> GPGSIPDYQEQDIFLWRKETGFGFRILGGNEPGEPIYIGHIVPLGAADTDGRLRSGDELICVDGTPVIGKSH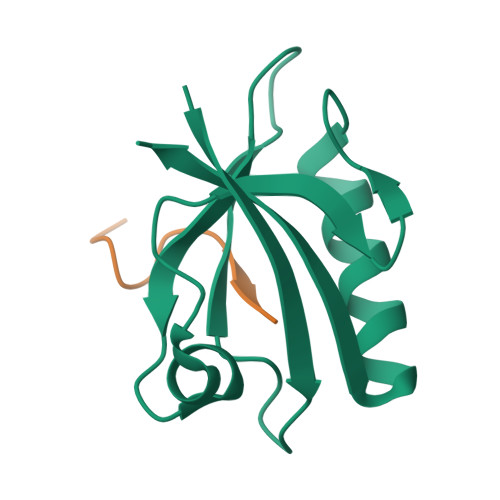QLVVQLMQQAAKQGHVNLTVRRKVV;> LPFELRGHLV> MSLTLGLR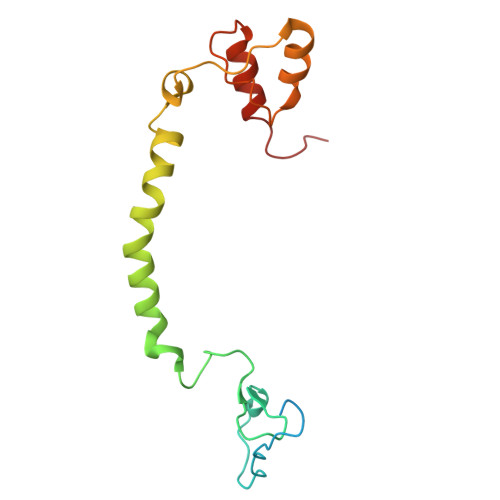SLSRGALAARNALPKRAGAGGPVKLSPPVDKPLPYNYDFWMDNGIYPGQPIYDGMFGSMVGNMSLEYMAKGWLVLLPILSAPFVYEHCIADDVTRNPFVPRQYPSEVREFLALFKNGFVLNDYSQPDYEEMKRRQSGLLTPIY>GSENLYFQSGAVARQERAIRTRQTILVAAAEVFDEVGYEAATISDVLKRSGVTKGALYFHFTSKQELAQAVLAEQVASLPRVPEQELKLQQSLDEALLLAHLLREGTGDPIVQGSVRLTVDQGSPRD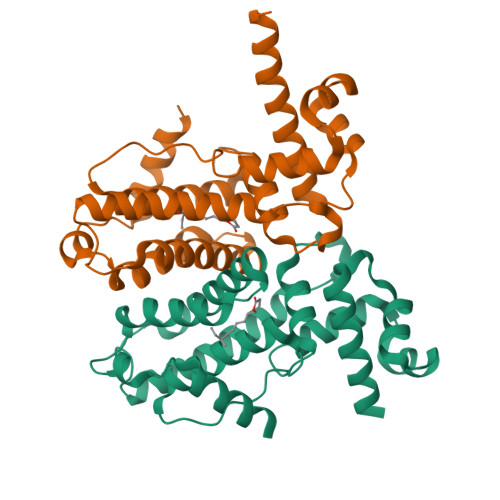HLNRRVPMQAWTEHTQSLFEEARAKGEILPHADVEALAKLFVGAFTGVQVLSRIMTGRADLAERVADLYRHLMPSFAMPGILVRLDFSPERGSRVYEAAMKQRESAAASTTDAARTLE[8x]> MSHIDDLAQLGTSTWLDDLSRERITSGNLSQVIEEKSVVGVTTNPAIFAA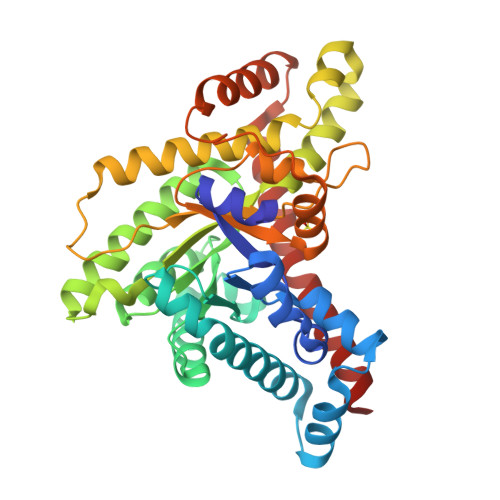AMSKGDSYDAQIAELKAAGASVDQAVYAMSIDDVRNACDLFTGIFESSNGYDGRVSIEVDPRISADRDATLAQAKELWAKVDRPNVMIKIPATPGSLPAITDALAEGISVNVTLIFSVARYREVIAAFIEGIKQAAANGHDVSKIHSVASFFVSRVDVEIDKRLEAIGSDEALALRGKAGVANAQRAYAVYKELFDAAELPEGANTQRPLWASTGVKNPAYAATLYVSELAGPNTVNTMPEGTIDAVLEQGNLHGDTLSNSAAEADAVFSQLEALGVDLADVFQVLETEGVDKFVASWSELLESMEARLK(2R)-2-amino-7-oxo-7-{[(2R,3S)-4,4,4-trifluoro-3-hydroxybutan-2-yl]amino}heptanoic 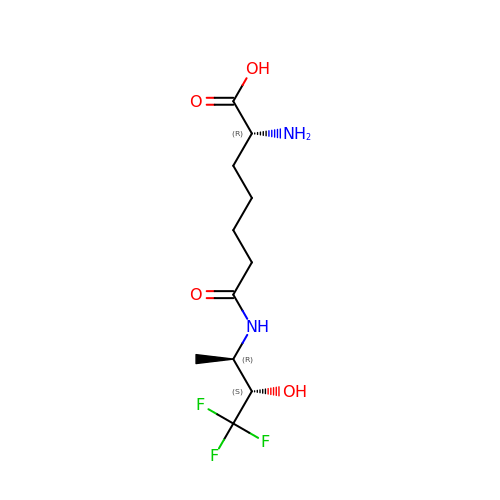acid | C11 H19 F3 N2 O4 | GCYIIHHJPYOBBJ-BHNWBGBOSA-N>[2x]GPHM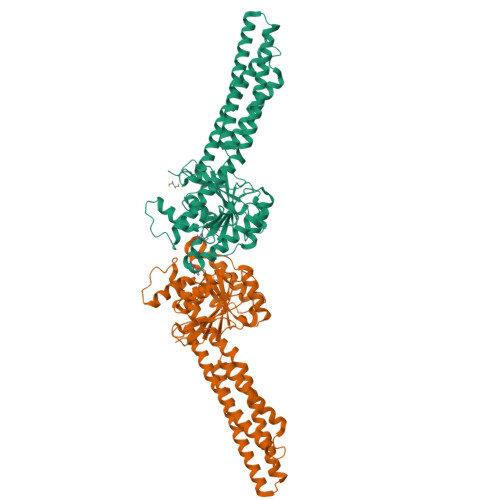GGSMAEPVSPLKHFVLAKKAITAIFDQLLEFVTEGSHFVEATYKNPELDRIATEDDLVEMQGYKDKLSIIGEVLSRRHMKVAFFGRTSSGKSSVINAMLWDKVLPSGIGHITNCFLSVEGTDGDKAYLMTEGSDEKKSVKTVNQLAHALHMDKDLKAGCLVRVFWPKAKCALLRDDLVLVDSPGTDVTTELDSWIDKFCLDADVFVLVANSESTLMNTEKHFFHKVNERLSKPNIFILNNRWDASASEPEYMEDVRRQHMERCLHFLVEELKVVNALEAQNRIFFVSAKEVLSARKQKAQGMPESGVALAEGFHARLQEFQNFEQIFEECISQSAVKTKFEQHTIRAKQILATVKNIMDSVNLAAEDKRHYSARLPKEIDQLEKIQNNSKLLRNKAVQLENELENFTKQFLPSSNEES>MATRSPGVVISDDEPGYDLDLFAIPNHYAEDLERVFIPHGLIMDRTERLARDVMKEMGGHHIVALCVLKGGYKFFADLLDYIKALNRNSDRSIPMTVDFIRLKSYANDQSTGDIKVIGGDDLSTLTGKNVLIVEDIIDTGKTMQTLLSLVRQYNPKMVKVASLLVKRTPRSVGYKPDFVGFEIPDKFVVGYALDYNEYFRDLNHVAVISETGKAKYKA[4x]

The key enzyme in the salvage pathway is hypoxanthine–guanine–(xanthine) phosphoribosyltransferase (HG(X)PRT)4. Inhibition of hypoxanthine–guanine–xanthine phosphoribosyltransferase activity decreases the pool of 6-oxo and 6-amino purine nucleoside monophosphates required for DNA and RNA synthesis, resulting in a reduction in cell growth. Five compounds synthesized here that contain a purine base covalently linked by a prolinol group to one or two phosphonate groups have Ki values ranging from 3 nM to >10 μM, depending on the structure of the inhibitor and the biological origin of the enzyme. X-ray crystal structures show that, on binding, these prolinol-containing inhibitors stimulated the movement of active site loops in the enzyme.

For the human enzyme, the l-prolinol and (R)-isomer configuration is the preferred configuration (i.e., 5). Key to this preference is the parallel π stacking of the purine base with the conserved aromatic amino acid in the enzyme (i.e., F186 in human HGPRT) and the fact that the 5′-phosphate pocket can expand to bind the 5′-phosphonate of 5. The phosphonate group of 5 does push further into this pocket than the phosphonate group of 1 or GMP, forcing the flexible loop (D137-T141) to move away. The movement of this loop triggers a further structural change, and this is between residues P168–V171. This loop also moves outward by approximately 1.7 Å. In human HGPRT, it is the phosphonate group attached to the carbon atom of the prolinol ring that enters the 5′-phosphate binding pocket whereas, when 5 is bound to TBrHGPRT1, it is the group that is attached to the nitrogen atom. In the human HGPRT·5 complex, the phosphonyl and carbonyl oxygens are coordinated to a magnesium ion and this sets up a network of bonds which firmly anchors this inhibitor in place. Superimposition of this complex onto that of the human enzyme in complex with the transition-state analogue, (1S)-1-(9-deazaguanyl-9-yl)-1,4-dideoxy-1,4-imino-d-ribitol 5-phosphate (ImmGP) together with pyrophosphate, shows that the phosphorus atom, the phosphonyl oxygens, and the carbonyl oxygen atoms of the inhibitor are located in a similar position as pyrophosphate. These interactions may be one of the most important features of this ligand that contribute to the nanomolar Ki values for human HGPRT (3 nM). The tail of the linker finds itself in a location that strongly mimics the location where pyrophosphate binds in the human ImmGP.PPi complex.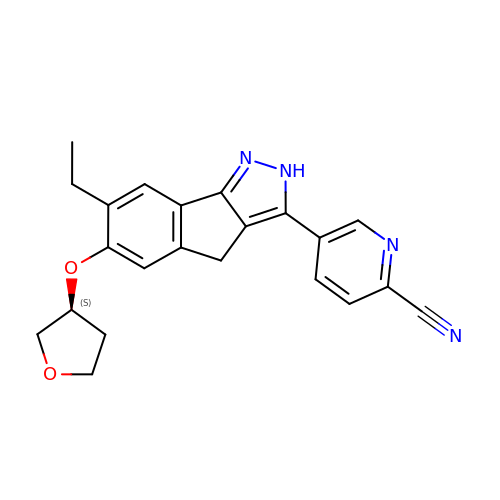5-{7-ethyl-6-[(3S)-tetrahydrofuran-3-yloxy]-2,4-dihydroindeno[1,2-c]pyrazol-3-yl}pyridine-2-carbonitrile | C22 H20 N4 O2 | OAWMFMUHXBYJGX-KRWDZBQOSA-N phenylazanium | C6 H8 N | 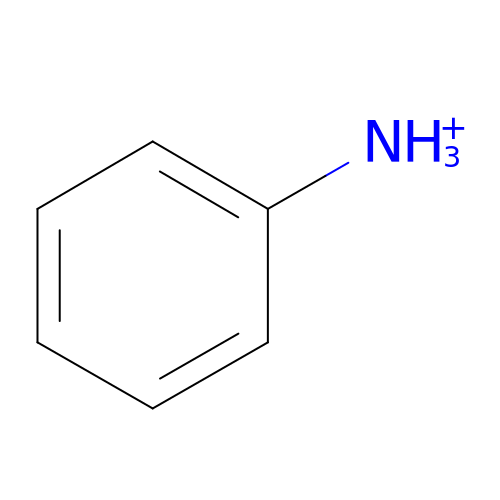PAYRUJLWNCNPSJ-UHFFFAOYSA-O>ARSEKRVPMTRLRKRVAERLLEAKNSTAMLTTFNEVNMKPIMDLRKQYGEAFEKRHGIRLGFMSFYVKAVVEALKRYPEVNASIDGDDVVYHNYFDVSMAVSTPRGLVTPVLRDVDTLGMADIEKKIKELAVKGRDGKLTVEDLTGGNFTITNGGVFGSLMSTPIINPPQSAILGMHAIKDRPMAVNGQVEILPMMYLALSYDHRLIDGRESVGFLVTIKELLEDPTRLLLDV[6x]

The second enzyme (E2) is a unique dihydro­lipo­amide succinyltransferase. To form an active complex, multiple copies of the E1 and E3 subunits attach to a core complex made of only E2 sub­units. One arrangement is made of 24 E2 subunits with an octahedral symmetry and the other is made of 60 E2 subunits with an icosahedral symmetry; both arrangements utilize trimers as building blocks. The E2 subunit contains three domains.

In our attempts to crystallize amidase (EC 3.5.1.4) from Arabidopsis thaliana (UniProt accession No. Q9FR37; Pollmann et al., 2003; Neu et al., 2007), we serendipitously crystallized the catalytic domain of E. coli dihydrolipoamide succinyltransferase (EC 2.3.1.61), which belongs to the family of α-keto acid dehydrogenase complexes, in a novel crystal form and without an expression tag. The structure lacks any observable electron density for the E3-binding domain, N-terminal lipoyl-binding domain or the associated linkers. It is likely that these domains are removed by endogenous proteases prior to or during the crystallization process. We have crystallized this enzyme in a new condition and in a new crystal form. The new crystallization precipitant contained only NaCl, which differs from the previously reported crystallization conditions as shown in Table 5. Even though EcDSCD is a well known highly crystallizable contaminant, its structure had never been reported in an I4 crystal form and SIMBAD did not find a hit when only searching the PDB unit-cell parameter database. Even in the I4 crystal form, the two trimers of the asymmetric unit adopt slightly different conformations, in which one trimer rotationally expands away around the threefold NCS axis of the trimer in comparison to the other trimer. Consequently, reconstruction of the 24-mer biological assembly using the asymmetric unit trimers and the fourfold crystallographic symmetry leads to a 24-mer that is slightly stretched outwards (skewed) compared with the 24-mer in the F432 form. Because of this conformational change, data in the I4 crystal form could not be processed in I422 and the packing is different from the previously reported F432 crystal form. Crystal-packing analysis shows an arrangement of a physiologically relevant 24-mer core complex in this structure, which provides additional insights into the organization of the E2 subunit of the E. coli KGDC.>MLNNAMSVVILAAGKGTRMYSDLPKVLHTLAGKAMVQHVIDAANELGAAHVHLVYGHGGDLLKQALKDDNLNWVLQAEQLGTGHAMQQAAP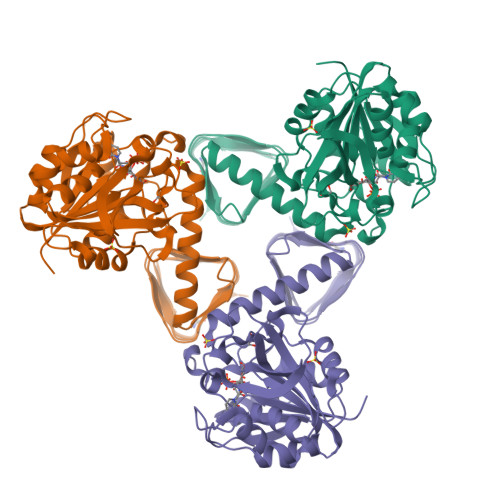FFADDEDILMLYGDVPLISVETLQRLRDAKPQGGIGLLTVKLDDPTGYGRITRENGKVTGIVEHKDATDEQRQIQEINTGILIANGADMKRWLAKLTNNNAQGEYYITDIIALAYQEGREIVAVHPQRLSEVEGVNNRLQLSRLERVYQSEQAEKLLLAGVMLRDPARFDLRGTLTHGRDVEIDTNVIIEGNVTLGHRVKIGTGCVIKNSVIGDDCEISPYTVVEDANLAAACTIGPFAR[2x]>MIVILDNGGQYVHRIHRSLKYIGVSSKIVPNTTPLEEIESNKEVKGIILSGGPDIEKAKNCIDIALNAKLPILGICLGHQLIALAYGGEVGRAEAEEYALTKVYVDKENDLFKNVPREFNAWASHKDEVKKVPEGFEILAHSDICQVEAMKHKTKPIYGVQFHPEVAHTEYGNEILKNFCKVCGY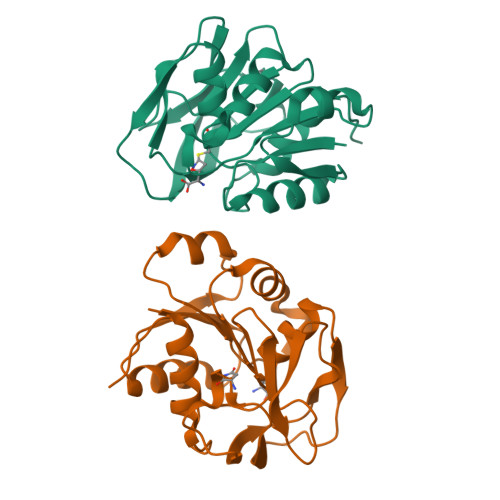KFE[2x]>[4x]MQNRQVANATKVAVAGASGYAGGEILRLLLGHPAYADGRLRIGALTAATSAGSTLGEHHPHLTPLAHRVVEPTEAAVLGGHDAVFLALPHGHSAVLAQQLSPETLIIDCGADFRLTDAAVWERFYGSSHAGSWPYGLPELPGARDQLR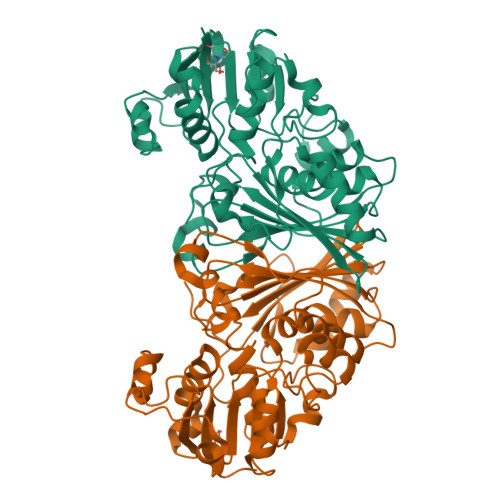GTRRIAVPGCYPTAALLALFPALAADLIEPAVTVVAVSGTSGAGRAATTDLLGAEVIGSARAYNIAGVHRHTPEIAQGLRAVTDRDVSVSFTPVLIPASRGILATCTARTRSPLSQLRAAYEKAYHAEPFIYLMPEGQLPRTGAVIGSNAAHIAVAVDEDAQTFVAIAAIDNLVKGTAGAAVQSMNLALGWPETDGLSVVGVAP> MTGSEIFLASKRAAITYDTDPATGEPRAWLAPGGTGNVVAEQAGVLNISWIASADSEDDRRASALNPDGVTMELHSGREILVRLIRHDPAVFRNVQNFMTANLMWAANNYGWDRWTQPSFGSDAREGWADFGRFTRDFADAILKSSAQSADPVYLVHDYQLVGVPALLREQRPDAPILLFVHIPWPSADYWRILPKEIRTGILHGMLPATTIGFFADRWCRNFLESVADLLPDARIDREAMTVEWRGHRTRLRTMPLGYSPLTLDGRNPQLPEGIEEWADGHRLVVHSGRTDPIKNAERAVRAFVLAARGGGLEKTRMLVRMNPNRLYVPANADYVHRVETAVAEANAELGSDTVRIDNDNDVNHTIACFRRADLLIFNSTVDGQNLSTFEAPLVNERDADVILSETCGAAEVLGEYCRSVNPFDLVEQAEAISAALA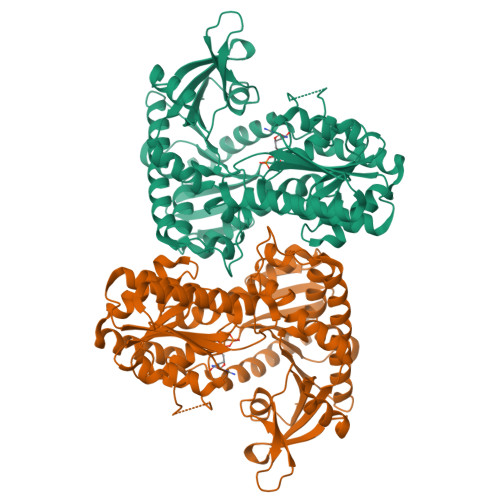AGPRQRAEAAARRRDAARPWTLEAWVQAQLDGLAADHAARTATAERFDTAPAVSTRADL>MHHHHHHGRIGIPRERLTNETRVAATPKTVEQLLKLGFTVAVESGAGQLASFDDKAFVQAGAEIVEGNSVWQSEIILKVNAPLDDEIALLNPGTTLVSFIWPAQNPELMQKLAERNVTVMAMDSVPRISRAQSLDALSSMANIAGYRAIVEAAHEFGRFFTGQITAAGKVPPAKVMVIGAGVAGLAAIGAANSLGAIVRAFDTRPEVKEQVQSMGAEFL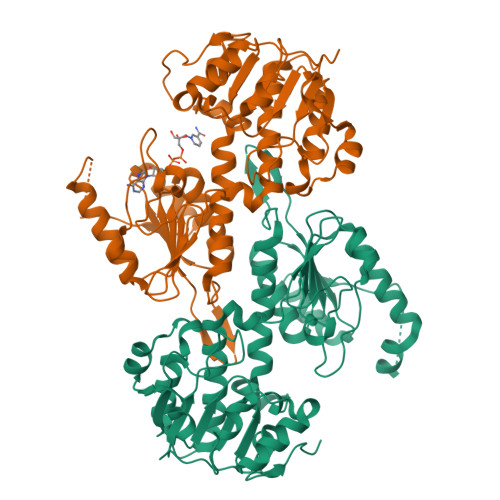ELDFKEEAGSGDGYAKVMSDAFIKAEMELFAAQAKEVDIIVTTALIPGKPAPKLITREMVDSMKAGSVIVDLAAQNGGNCEYTVPGEIFTTENGVKVIGYTDLPGRLPTQSSQLYGTNLVNLLKLLCKEKDGNITVDFDDVVIRGVTVIRAGEITWPAPPIQVSAQPQAAQKAAPEVKTEEK[2x]>GSKGLENPLPERPREKEEPVVRETGEVVDCHLSDMLQQLHSVNASKPSERGLVRQEEAEDPACIPIFWVSKWVDYSDKYGLGYQLCDNSVGVLFNDSTRLILYNDGDSLQYIERDGTESYLTVSSHPNSLMKKITLLKYFRNYMSEHLLKAGANITPREGDELARLPYLRTWFRT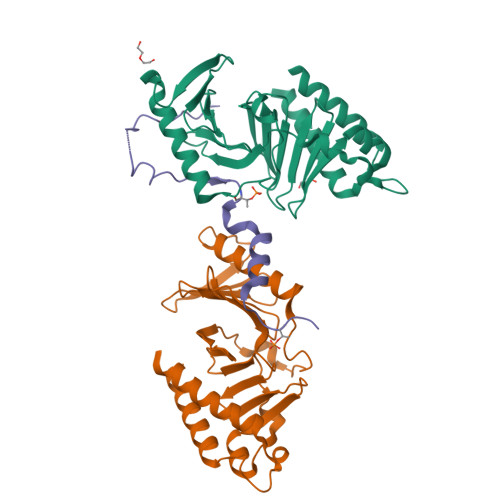RSAIILHLSNGSVQINFFQDHTKLILCPLMAAVTYIDEKRDFRTYRLSLLEEYGCCKELASRLRYARTMVDKLLSSRSASNRLKAS[2x];> GSKPIDVFDFPDNSDVSSIGRLGENEKDEETYETFDPPLHSTAIYADEEEFSKHCGLSLSSTPPGKEAKRSSDTSGNE> MGSSHHHHHHHSSGRENLYFQGHMEGVRWAFSCGTWLPSRAEWLLAVRSIQPEEKERIGQFVFARDAKAAMAGRLMIRKLVAEKLNIPWNHIRLQRTAKGKPVLAKDSSNPYPNFNFNISHQGDYAVLAAEPELQVGIDIMKTSFPGRGSIPEFFHIMKRKFTNKEWETIRSFKDEWTQLDMFYRNWALKESFIKAIGVGLGFELQRLEFDLSPLNLDIGQVYKETRLFLDGEEEKEWAFEESKIDEHHFVAVALRKPDGSRHQDVPSQDDSKPTQRQFTILNFNDLMSSAVPMTPEDPSFWDCFCFTEEIPIRNGTKSLESG

The posttranslational modification of a conserved serine residue in carrier proteins with a phosphopantetheinyl moiety transferred from coenzyme A through the enzyme phosphopantetheinyl transferase (PPT) is vital to all living organisms. Molecular cloning and biochemical characterization of human PPT revealed that this cytosolic enzyme is a Mg2+-requiring monomeric enzyme that exhibits a broad acceptor substrate specificity. Whereas microbial genomes contain more than one PPT, only one PPT has been identified in mammals. This enzyme exhibits a broad substrate specificity and is able to phosphopantetheinylate the ACP components of the cytosolic and the mitochondrial FAS systems, as well as aminoadipate semialdehyde dehydrogenase, the human ortholog to the yeast lys5 gene. Human phosphopantetheinyl transferase exhibits an α/β fold and 2-fold pseudosymmetry similar to the Sfp phosphopantetheinyl transferase from Bacillus subtilis.

CoA is bound in a bent conformation with the pyrophosphate group at the apex of the bend, and clear density is observed for all parts of the molecule including the phosphopantheteinyl moiety. The 3-phospho-adenosine portion of CoA is tightly bound through a combination of hydrophobic and hydrogen-bonding interactions contributed by residues Lys89, Lys91, Asn108, Arg47, and Arg86. The latter two basic residues play a key role by forming salt bridges to the oxygen atoms of the 3′-phosphate of the adenine ribose. In addition, the Nɛ2 nitrogen of the imidazole side chain of His111 binds to the 3′-phosphate group. The α-phosphate group of the pyrophosphate moiety is held in place by interactions with the main-chain amide of His111 and the side-chain hydroxyl of Ser110, while the phosphopantheteinyl group is bound through interactions with side and main chains of residues Glu181, Gly190, Leu191, and Leu195. Magnesium is coordinated by the α and β groups of the CoA pyrophosphate, the carboxylates of Asp129 and Glu181, and one water molecule. A sixth ligand for the Mg is not present in the final crystallographic model; however, there is some residual density that implies this position may be occupied by a poorly ordered water molecule. The metal cation is found in a solvent inaccessible area, shielded by protein and CoA moieties. As found in many other Mg binding proteins, PPT has, besides the inner coordination sphere of the ligands described above, a hydrophobic outer shell that is provided by residues Ile130, Met131, Tyr174, and Trp177, thus creating an environment of high hydrophobic contrast. In the PPT-CoA complex, the long C-terminal coil of the enzyme (residues 290–305) is highly ordered due to its participation in crystal packing with two other subunits in the crystal lattice.8-(naphthalen-1-yl)-6-(1H-pyrrol-2-yl)quinoline-2-carboxylic acid | C24 H16 N2 O2 | 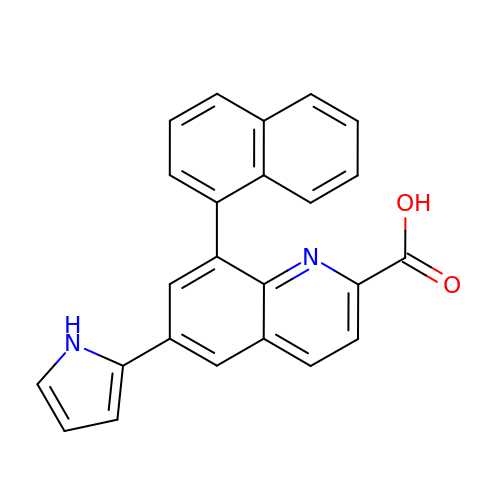RSHSGQQZDAKAOC-UHFFFAOYSA-N>[4x]GSMATSTSTSTPIIFYDIAQRPPVAETCCAPNPWKSRLALNFKAVPYTTTWVKLPDIERVCKEIGAEPSAFGLLKEGKPYYTLPIIHDPATDSLIGDSFDIAAYLQRTYPASGAGDLFPPQKLDYAVGRDMQQLLFPLSEIRASPELADYARFNSNVDAAFTAHVGLMVHGLPLDPATAEVTKAEFVRRAGLSSWDDLEMVGEARDKMMQSFRNMLGDLAALFRKDASGPFLLGQRA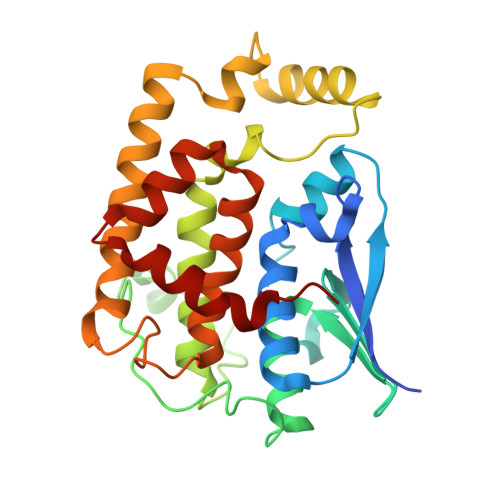TYADMIVGGWLRMMRATLPVSEWQEARAWHGGIFGRLHDALDKYAEVK>GSHMDNQCTVQVRLELGHRAQLRKKPTTEGFTHDWMVFVRGPEQCDIQHFVEKVVFWLHDSFPKPRRVCKEPPYKVEESGYAGFIMPIEVHFKNKEEPRKVCFTYDLFLNLEGNPPVNHLNHLRCEKLT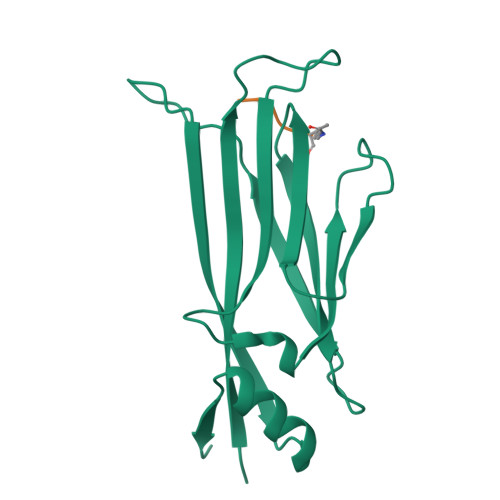FNNPTTEFRYKLLRAGGVMVMPEGAHHHHHH[2x];>AARK[2x]>MSEEQSHADQDAYVADVDGILDVLRAQVLERKPDDIFQFISKSALSLQKDRGAESCDRINCKVKDEQKSRALTIIVFGASGDLAKKKTFPALFDLYCGGLLPPEVNIIGYARTKVDDVEKWKHETLMKYFSNLSERGCHAEDFLKHISYFCGAYDSVDDFKRLDAVIREKENAFKGPEKGGNRLFYLALPPSVFASVCESIHKGAMPQEVGGWVRVIIEKPFGRDTKSSAELSQALEPFFDESQLYRIDHYLGKEMVQNIITTRFANRIFSAVWNASNIACVQITFKETIGTEGRGGYFDNIGIIRDVMQNHLTQILALLAMEKPRSLDAECIRDEKVSVLKCIEPITKENCVLGQYTASADGSIPGYLEDVTVPEGSTCPTFAVMRLNINNDRWAGVPFILKAGKAVEQKYVAIRIQFRDEVHPYGEATQRNELVIRAQPSEAMYVKITTKVPGLSGDLRQTHQTELDLTYHTRYDVRLPDAYESLINDALLGNSTNFVRKDELDVAWRIFTPLLHQIDSGEIKPI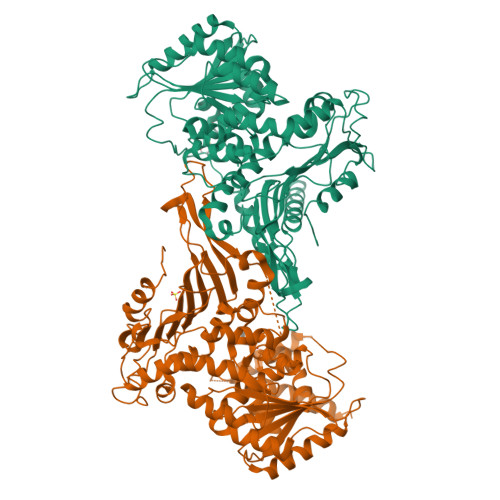PYQAGTRGPKEADEFIANNGFKHQKGYHWLPSNKL[2x]>MSLESLTVQTKYGPVRGKRSVSLLGQEYVSFQGIPYARAPEGELRFKAPVPPQNWTETLDCSQQCEPCYHFDRRLQKIVGCEDSLKINVFAKEINPSKPLPVMLYIYGGGFTEGTSGTELYGPDFLVQKDIVLVSFNYRIGALGFLCCQSEQDGVPGNAGLKDQNLAIRWVLENIAAFGGDPKRVTLVGHSAGAASVQYHLISDASKDLFQRAIVMSGSTYNSWSLTRQRNWVEKLAKAIGWDGQGGESG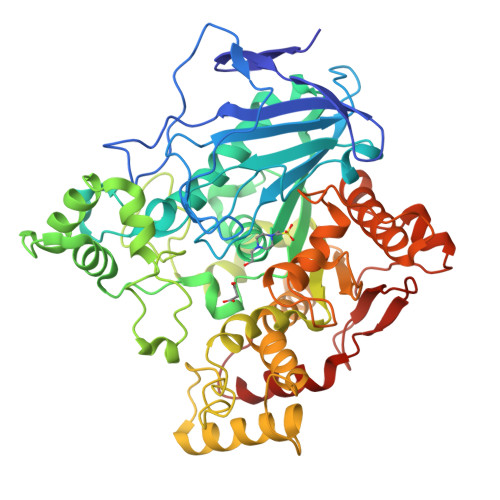ALRFLKAAKPEDIVANQEKLLTDQDMQDDIFTPFGPTVEPYLTEQCMIPKEPFEMARTAWGDKIDIMIGGTSEEGLLLLQKIKLQPELLSHPHLFLGNVPPNLKISMEKRIEFAAKLKQRYYPDSSPSMENNLGYVHMMSDRVFWHGLHRTILARAARSRARTFVYRICLDSEFYNHYRIMMIDPKLRGTAHADELSYLFSNFTQQVPGKETFEYRGLQTLVDVFTAFVINGDPNCGMTAKSGVVFEPNAQTKPTFKCLNIANDGVAFVDYPDADRLDMWDAMYVNDELF[2x]>GAINKNMKLGQKVLIPVKQFPKFNFVGKLLGPRGNSLKRLQEETLTKMSILGKGSMRDKAKEEELRKSGEAKYFHLNDDLHVLIEVFAPPAEAYARMGHALEEIKKFLIPDYN[6x]

T-STAR is a tissue-specific STAR protein mainly expressed in the testis and brain3426, and regulates the alternative splicing of CD44, Tra2β, Tau, VGEF and Neurexin pre-mRNAs262728. STAR proteins are defined by the presence of a highly conserved RNA-binding domain, the STAR domain, also responsible for homodimerization, and composed of a central KH (K homology) domain flanked by two highly conserved regions, QUA1 and QUA2. Here, we have determined the X-ray structures of the T-STAR KH domain in its free state, and in complex with AAAUAA; KH-QUA2 in complex with AAUAAU; QUA1-KH in complex with UAAU; and the full STAR domain in complex with AUUAAA. Taken together, our data reveal a unique mode of RNA recognition and dimerization by the STAR proteins Sam68 and T-STAR that is crucial for their function in alternative splicing.

All our structures of T-STAR in complex with RNA display a very similar mode of RNA recognition, and show that the KH domain specifically recognizes three nucleotides with the sequences U1A2A3 or A1A2A3 as illustrated for the structure of T-STAR KH-AAAUAA where one KH domain binds the 5′-AAA and another KH binds the 3′-UAA moieties of the RNA. The RNA lies in the classical KH hydrophobic groove that comprises α-helices 1 and 2, β-strand 2, the GXXG loop and the variable loop4647. The base of the nucleotide A3 is specifically recognized through intermolecular hydrogen bonds with the backbone atoms of I97 in β-strand 2 mimicking a Watson-Crick base pair. The base of the nucleotide A2 is specifically recognized through an intermolecular hydrogen bond to N71 side chain. Finally, the nucleotide A1 or U1 is stabilized by van der Walls contacts to G74, K75 and G78 of helix 1, and A1 is stabilized by a hydrogen bond to the side chain of D158 at the C-terminus of the KH domain. Additional nucleotides located 5′ or 3′ of the (A/U)AA motif are visible in our structures but do not make specific contacts to the protein, suggesting that only the (A/U)AA motif is specifically recognized by T-STAR. All the KH-RNA contacts observed in the X-ray structures are consistent with NMR chemical shift perturbation experiments showing that the residues of T-STAR KH and Sam68 STAR that display the largest chemical shift perturbations upon RNA binding correspond to the residues that contact the RNA in the X-ray structures. A comparison of free and RNA-bound structures of T-STAR show that the presence of the QUA1, QUA2 and the RNA do not induce any global structural changes of the KH domain (backbone RMSD ranging between 0.44 and 1.05 Å).1~{H}-benzimidazol-2-ylcyanamide | C8 H6 N4 | 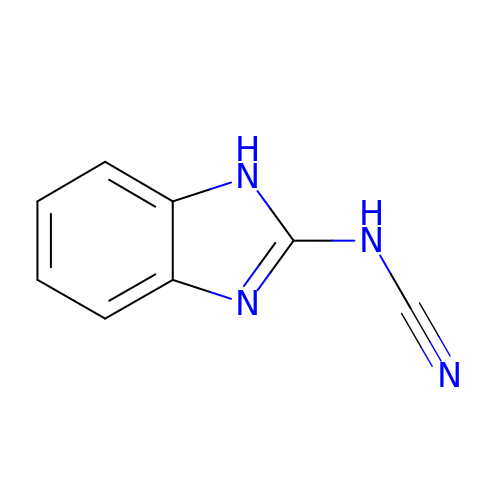NYLIXUBOFQIMGV-UHFFFAOYSA-N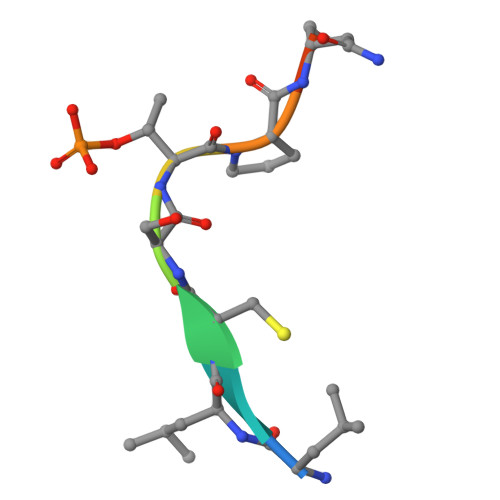> LLCSTPNGL2-[(6R)-6-(dioxidanyl)-6-oxidanyl-3-oxidanylidene-cyclohexa-1,4-dien-1-yl]ethanoic 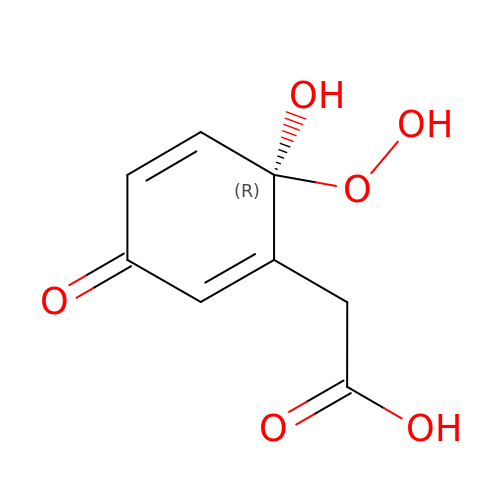acid | C8 H8 O6 | WRLJTDRVSAMRQB-MRVPVSSYSA-N>LKLSAENESTPIQQLLEHFLRQLQRKDPHGFFAFPVTDAIAPGYSMIIKHPMDFGTMKDKIVANEYKSVTEFKADFKLMCDNAMTYNRPDTVYYKLAKKILHAGFKMMSKERLLA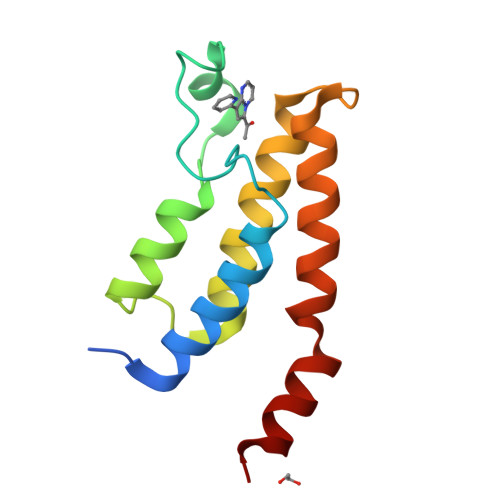LKRSMS[2x]> MSQDRILLDLDVVNQRLILFNSAFPSDAIEAPFHFSNKESTSENLDNLAGTILHSRSITGHVFLYKHIFLEIVARWIKDSKKKDYVLVIEKLASIITIFPVAMPLIEDYLDKENDHFITILQNPSTQKDSDMFKILLAYYRLLYHNKEVFARFIQPDILYQLVDLLTKEQENQVVIFLALKVLSLYLDMGEKTLNDMLDTYIKSRDSLLGHFEGDSGIDYSFLELNEAKRCANFSKLPSVPECFTIEKKSSYFIIEPQDLSTKVASICGVIVPKVHTIHDKVFYPLTFVPTHKTVSSLRQLGRKIQNSTPIMLIGKAGSGKTFLINELSKYMGCHDSIVKIHLGEQTDAKLLIGTYTSGDKPGTFEWRAGVLATAVKEGRWVLIEDIDKAPTDVLSILLSLLEKRELTIPSRGETVKAANGFQLISTVRINEDHQKDSSNKIYNLNMIGMRIWNVIELEEPSEEDLTHILAQKFPILTNLIPKLIDSYKNVKSIYMNTKFISLNKGAHTRVVSVRDLIKLCERLDILFKNNGINKPDQLIQSSVYDSIFSEAADCFAGAIGEFKALEPIIQAIGESLDIASSRISLFLTQHVPTLENLDDSIKIGRAVLLKEKLNIQKKSMNSTLFAFTNHSLRLMEQISVCIQMTEPVLLVGETGTGKTTVVQQLAKMLAKKLTVINVSQQTETGDLLGGYKPVNSKTVAVPIQENFETLFNATFSLKKNEKFHKMLHRCFNKNQWKNVVKLWNEAYKMAQSILKITNTENENENAKKKKRRLNTHEKKLLLDKWADFNDSVKKFEAQSSSIENSFVFNFVEGSLVKTIRAGEWLLLDEVNLATADTLESISDLLTEPDSRSILLSEKGDAEPIKAHPDFRIFACMNPATDVGKRDLPMGIRSRFTEIYVHSPERDITDLLSIIDKYIGKYSVSDEWVGNDIAELYLEAKKLSDNNTIVDGSNQKPHFSIRTLTRTLLYVTDIIHIYGLRRSLYDGFCMSFLTLLDQKSEAILKPVIEKFTLGRLKNVKSIMSQTPPSPGPDYVQFKHYWMKKGPNTIQEQAHYIITPFVEKNMMNLVRATSGKRFPVLIQGPTSSGKTSMIKYLADITGHKFVRINNHEHTDLQEYLGTYVTDDTGKLSFKEGVLVEALRKGYWIVLDELNLAPTDVLEALNRLLDDNRELFIPETQEVVHPHPDFLLFATQNPPGIYGGRKILSRAFRNRFLELHFDDIPQDELEIILRERCQIAPSYAKKIVEVYRQLSIERSASRLFEQKNSFATLRDLFRWALRDAVGYEQLAASGYMLLAERCRTPQEKVTVKKTLEKVMKVKLDMDQYYASLEDKSLEAIGSVTWTKGMRRLSVLVSSCLKNKEPVLLVGETGCGKTTICQLLAQFMGRELITLNAHQNTETGDILGAQRPVRNRSEIQYKLIKSLKTALNIANDQDVDLKELLQLYSKSDNKNIAEDVQLEIQKLRDSLNVLFEWSDGPLIQAMRTGNFFLLDEISLADDSVLERLNSVLEPERSLLLAEQGSSDSLVTASENFQFFATMNPGGDYGKKELSPALRNRFTEIWVPSMEDFNDVNMIVSSRLLEDLKDLANPIVKFSEWFGKKLGGGNATSGVISLRDILAWVEFINKVFPKIQNKSTALIQGASMVFIDALGTNNTAYLAENENDLKSLRTECIIQLLKLCGDDLELQQIETNEIIVTQDELQVGMFKIPRFPDAQSSSFNLTAPTTASNLVRVVRAMQVHKPILLEGSPGVGKTSLITALANITGNKLTRINLSEQTDLVDLFGADAPGERSGEFLWHDAPFLRAMKKGEWVLLDEMNLASQSVLEGLNACLDHRGEAYIPELDISFSCHPNFLVFAAQNPQYQGGGRKGLPKSFVNRFSVVFIDMLTSDDLLLIAKHLYPSIEPDIIAKMIKLMSTLEDQVCKRKLWGNSGSPWEFNLRDTLRWLKLLNQYSICEDVDVFDFVDIIVKQRFRTISDKNKAQLLIEDIFGKFSTKENFFKLTEDYVQINNEVALRNPHYRYPITQNLFPLECNVAVYESVLKAINNNWPLVLVGPSNSGKTETIRFLASILGPRVDVFSMNSDIDSMDILGGYEQVDLTRQISYITEELTNIVREIISMNMKLSPNATAIMEGLNLLKYLLNNIVTPEKFQDFRNRFNRFFSHLEGHPLLKTMSMNIEKMTEIITKEASVKFEWFDGMLVKAVEKGHWLILDNANLCSPSVLDRLNSLLEIDGSLLINECSQEDGQPRVLKPHPNFRLFLTMDPKYGELSRAMRNRGVEIYIDELHSRSTAFDRLTLGFELGENIDFVSIDDGIKKIKLNEPDMSIPLKHYVPSYLSRPCIFAQVHDILLLSDEEPIEESLAAVIPISHLGEVGKWANNVLNCTEYSEKKIAERLYVFITFLTDMGVLEKINNLYKPANLKFQKALGLHDKQLTEETVSLTLNEYVLPTVSKYSDKIKSPESLYLLSSLRLLLNSLNALKLINEKSTHGKIDELTYIELSAAAFNGRHLKNIPRIPIFCILYNILTVMSENLKTESLFCGSNQYQYYWDLLVIVIAALETAVTKDEARLRVYKELIDSWIASVKSKSDIEITPFLNINLEFTDVLQLSRGHSITLLWDIFRKNYPTTSNSWLAFEKLINLSEKFDKVRLLQFSESYNSIKDLMDVFRLLNDDVLNNKLSEFNLLLSKLEDGINELELISNKFLNKRKHYFADEFDNLIRYTFSVDTAELIKELAPASSLATQKLTKLITNKYNYPPIFDVLWTEKNAKLTSFTSTIFSSQFLEDVVRKSNNLKSFSGNQIKQSISDAELLLSSTIKCSPNLLKSQM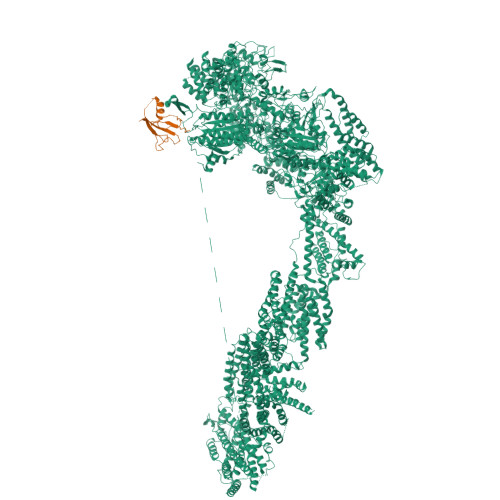EYYKNMLLSWLRKVIDIHVGGDCLKLTLKELCSLIEEKTASETRVTFAEYIFPALDLAESSKSLEELGEAWITFGTGLLLLFVPDSPYDPAIHDYVLYDLFLKTKTFSQNLMKSWRNVRKVISGDEEIFTEKLINTISDDDAPQSPRVYRTGMSIDSLFDEWMAFLSSTMSSRQIKELVSSYKCNSDQSDRRLEMLQQNSAHFLNRLESGYSKFADLNDILAGYIYSINFGFDLLKLQKSKDRASFQISPLWSMDPINISCAENVLSAYHELSRFFKKGDMEDTSIEKVLMYFLTLFKFHKRDTNLLEIFEAALYTLYSRWSVRRFRQEQEENEKSNMFKFNDNSDDYEADFRKLFPDYEDTALVTNEKDISSPENLDDIYFKLADTYISVFDKDHDANFSSELKSGAIITTILSEDLKNTRIEELKSGSLSAVINTLDAETQSFKNTEVFGNIDFYHDFSIPEFQKAGDIIETVLKSVLKLLKQWPEHATLKELYRVSQEFLNYPIKTPLARQLQKIEQIYTYLAEWEKYASSEVSLNNTVKLITDLIVSWRKLELRTWKGLFNSEDAKTRKSIGKWWFYLYESIVISNFVSEKKETAPNATLLVSSLNLFFSKSTLGEFNARLDLVKAFYKHIQLIGLRSSKIAGLLHNTIKFYYQFKPLIDERITNGKKSLEKEIDDIILLASWKDVNVDALKQSSRKSHNNLYKIVRKYRDLLNGDAKTIIEAGLLYSNENKLKLPTLKQHFYEDPNLEASKNLVKEISTWSMRAAPLRNIDTVASNMDSYLEKISSQEFPNFADLASDFYAEAERLRKETPNVYTKENKKRLAYLKTQKSKLLGDALKELRRIGLKVNFREDIQKVQSSTTTILANIAPFNNEYLNSSDAFFFKILDLLPKLRSAASNPSDDIPVAAIERGMALAQSLMFSLITVRHPLSEFTNDYCKINGMMLDLEHFTCLKGDIVHSSLKANVDNVRLFEKWLPSLLDYAAQTLSVISKYSATSEQQKILLDAKSTLSSFFVHFNSSRIFDSSFIESYSRFELFINELLKKLENAKETGNAFVFDIIIEWIKANKGGPIKKEQKRGPSVEDVEQAFRRTFTSIILSFQKVIGDGIESISETDDNWLSASFKKVMVNVKLLRSSVVSKNIETALSLLKDFDFTTTESIYVKSVISFTLPVITRYYNAMTVVLERSRIYYTNTSRGMYILSTILHSLAKNGFCSPQPPSEEVDDKNLQEGTGLGDGEGAQNNNKDVEQDEDLTEDAQNENKEQQDKDERDDENEDDAVEMEGDMAGELEDLSNGEENDDEDTDSEEEELDEEIDDLNEDDPNAIDDKMWDDKASDNSKEKDTDQNLDGKNQEEDVQAAENDEQQRDNKEGGDEDPNAPEDGDEEIENDENAEEENDVGEQEDEVKDEEGEDLEANVPEIETLDLPEDMNLDSEHEESDEDVDMSDGMPDDLNKEEVGNEDEEVKQESGIESDNENDEPGPEEDAGETETALDEEEGAEEDVDMTNDEGKEDEENGPEEQAMSDEEELKQDAAMEENKEKGGEQNTEGLDGVEEKADTEDIDQEAAVQQDSGSKGAGADATDTQEQDDVGGSGTTQNTYEEDQEDVTKNNEESREEATAALKQLGDSMKEYHRRRQDIKEAQTNGEEDENLEKNNERPDEFEHVEGANTETDTQALGSATQDQLQTIDEDMAIDDDREEQEVDQKELVEDADDEKMDIDEEEMLSDIDAHDANNDVDSKKSGFIGKRKSEEDFENELSNEHFSADQEDDSEIQSLIENIEDNPPDASASLTPERSLEESRELWHKSEISTADLVSRLGEQLRLILEPTLATKLKGDYKTGKRLNMKRIIPYIASQFRKDKIWLRRTKPSKRQYQIMIALDDSKSMSESKCVKLAFDSLCLVSKTLTQLEAGGLSIVKFGENIKEVHSFDQQFSNESGARAFQWFGFQETKTDVKKLVAESTKIFERARAMVHNDQWQLEIVISDGICEDHETIQKLVRRARENKIMLVFVIIDGITSNESILDMSQVNYIPDQYGNPQLKITKYLDTFPFEFYVVVHDISELPEMLSLILRQYFTDLASS;> MSTLIPPPSKKQKKEAQLPREVAIIPKDLPNVSIKFQALDTGDNVGGALRVPGAISEKQLEELLNQLNGTSDDPVPYTFSCTIQGKKASDPVKTIDITDNLYSSLIKPGYNSTEDQITLLYTPRAVFKVKPVTRSSSAIAGHGSTILCSAFAPHTSSRMVTGAGDNTARIWDCDTQTPMHTLKGHYNWVLCVSWSPDGEVIATGSMDNTIRLWDPKSGQCLGDALRGHSKWITSLSWEPIHLVKPGSKPRLASSSKDGTIKIWDTVSRVCQYTMSGHTNSVSCVKWGGQGLLYSGSHDRTVRVWDINSQGRCINILKSHAHWVNHLSLSTDYALRIGAFDHTGKKPSTPEEAQKKALENYEKICKKNGNSEEMMVTASDDYTMFLWNPLKSTKPIARMTGHQKLVNHVAFSPDGRYIVSASFDNSIKLWDGRDGKFISTFRGHVASVYQVAWSSDCRLLVSCSKDTTLKVWDVRTRKLSVDLPGHKDEVYTVDWSVDGKRVCSGGKDKMVRLWTH> MGGSEVGTVPVTWRLGVDVGERSIGLAAVSYEEDKPKEILAAVSWIHDGGVGDERSGASRLALRGMARRARRLRRFRRARLRDLDMLLSELGWTPLPDKNVSPVDAWLARKRLAEEYVVDETERRRLLGYAVSHMARHRGWRNPWTTIKDLKNLPQPSDSWERTRESLEARYSVSLEPGTVGQWAGYLLQRAPGIRLNPTQQSAGRRAELSNATAFETRLRQEDVLWELRCIADVQGLPEDVVSNVIDAVFCQKRPSVPAERIGRDPLDPSQLRASRACLEFQEYRIVAAVANLRIRDGSGSRPLSLEERNAVIEALLAQTERSLTWSDIALEILKLPNESDLTSVPEEDGPSSLAYSQFAPFDETSARIAEFIAKNRRKIPTFAQWWQEQDRTSRSDLVAALADNSIAGEEEQELLVHLPDAELEALEGLALPSGRVAYSRLTLSGLTRVMRDDGVDVHNARKTCFGVDDNWRPPLPALHEATGHPVVDRNLAILRKFLSSATMRWGPPQSIVVELGGGSAGGYAAVALRDRLLSYGEKNGVAQVAVFRGGVTAEARRWLDISIERLFSRVAIFAQSTSTKRLDRRHHAVDAVVLTTLTPGVAKTLADARSRRVSAEFWRRPSDVNRHSTEEPQSPAYRQWKESCSGLGDLLISTAARDSIAVAAPLRLRPTGALHEETLRAFSEHTVGAAWKGAELRRIVEPEVYAAFLALTDPGGRFLKVSPSEDVLPADENRHIVLSDRVLGPRDRVKLFPDDRGSIRVRGGAAYIASFHHARVFRWGSSHSPSFALLRVSLADLAVAGLLRDGVDVFTAELPPWTPAWRYASIALVKAVESGDAKQVGWLVPGDELDFGPEGVTTAAGDLSMF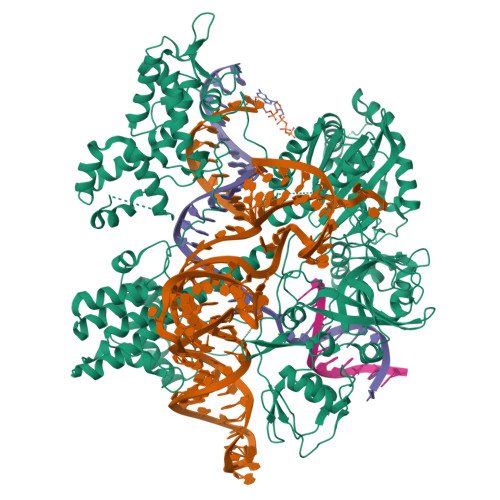LKYFPERHWVVTGFEDDKRINLKPAFLSAEQAEVLRTERSDRPDTLTEAGEILAQFFPRCWRATVAKVLCHPGLTVIRRTALGQPRWRRGHLPYSWRPWSADPWSGGTPHHHHHH> QAQITGRPEWIWLALGTALMGLGTLYFLVKGMGVSDPDAKKFYAIVTLVPAIAFTMYLSMLLGYGLTMVPFGGEQNPIYWARYADWLFTTPLLLLDLALLVDADQGTILALVGADGIMIGTGLVGALTKVYSYRFVWWAISTAAMLYILYVLFFGFTSKAESMRPEVASTFKVLRNVTVVLWSAYPVVWLIGSEGAG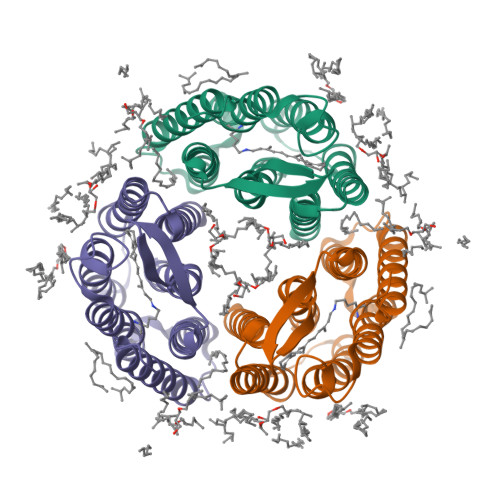IVPLNIETLLFMVLDVSAKVGFGLILLRSRAIFGEAEAPEPSAGDGAAATSD>[14x]MSFPYFISPEQAMRERSELARKGIARAKSVVALAYAGGVLFVAENPSRSLQKISELYDRVGFAAAGKFNEFDNLRRGGIQFADTRGYAYDRRDVTGRQLANVYAQTLGTIFTEQAKPYEVELCVAEVAHYGETKRPELYRIT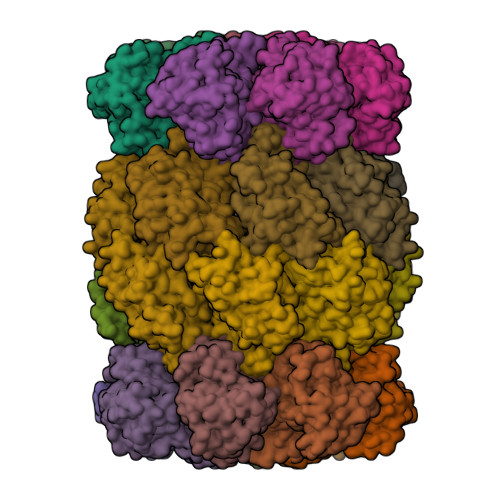YDGSIADEPHFVVMGGTTEPIANALKESYAENASLTDALRIAVAALRAGSADTSGGDQPTLGVASLEVAVLDANRPRRAFRRITGSALQALLVDQESPQSDGESSG;>ATIVALKYPGGVVMAGDRRSTQGNMISGRDVRKVYITDDYTATGIAGTAAVAVEFARLYAVELEHYEKLEGVPLTFAGKINRLAIMVRGNLAAAMQGLLALPLLAGYDIHASDPQSAGRIVSFDAAGGWNIEEEGYQAVGSGSLFAKSSMKKLYSQVTDGDSGLRVAVEALYDAADDDSATGGPDLVRGIFPTAVIIDADGAVDVPESRIAELARAIIESRSGADTFGSDGGEK[14x]> MRGSHHHHHHGRSRSLNPLSTPQFDSTDETPASYNLAVRRAAPAVVNVYNRGLNTNSHNQLEIRTLGSGVIMDQRGYIITNKHVINDADQIIVALQDGRVFEALLVGSDSLTDLAVLKINATGGLPTIPI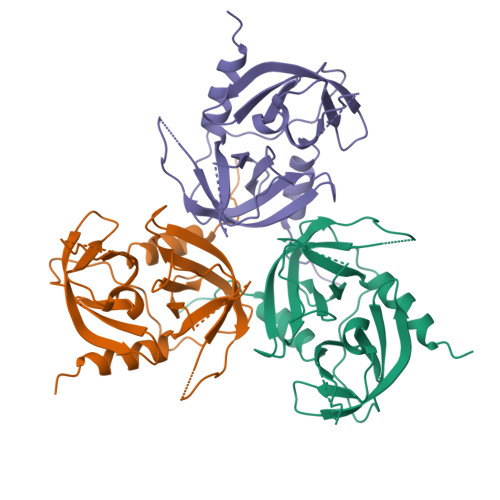NARRVPHIGDVVLAIGNPYNLGQTITQGIISATGRIGLNPTGRQNFLATDASINHGNSGGALVNSLGELMGINTLSFDKSNDGETPEGIGFAIPFQLATKIMDKLIRDGRVIR>[2x]GIDPFTQRNAIREDLDNYLNEMGEVTADNIQTWLSGRILLIENAAQNIAINPEPAAVASLLEQKA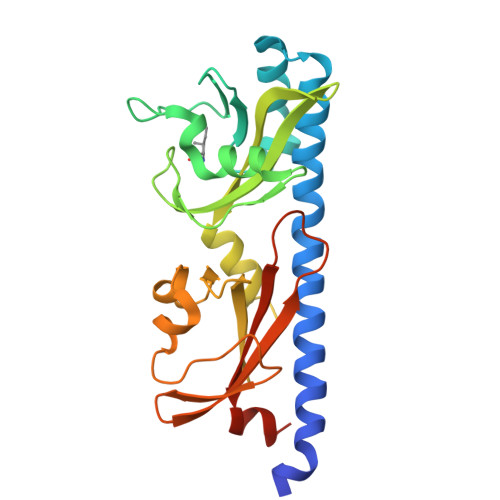LTSTFMASYLGDATGHFTIRPDAKMPDGFDPRVRPWYKGAESSSTSTLTEPYIDAATGQTIISIATAAKKAGQSVGVVGGDLSLQTLINTLSARDFSGMGYAFLVSADGKILVHPDKALVMKSLKEAYPQDTPRISSDFSEVTVDGKTRIVNFTPIKGLPSVNWYIGLSVDKDKAFSMLSEFRTS> MKIMKEFKEQFGYQLSNFDDMDIKGYANLYQKDIGKDVSMIEQGLKQLSITETEVLLPEQINKKLLGVLNMNEVNQSSNTWVGTLTKQLVSSENNFNIQELPTARKEVFKELLVNRELPQTLRDVITITDDEHVESIPALSYIKDKLATNGIELSLNGSSKYFDRREGHIYTEVADSVVHGSDRTLDDLLKEIFINECVSYETTLLLDKNNASGLIDKDNQDLSLYNQGIKEVSNTSMYDGIKQAMKDIPQTFRRKVSVVMNTEHHDKLIKELAQMGLGTLAGDLTKLFNVSHVVVTDDAQDIFVGDFGHAIYAKYEPIMYNKKKQALKGVYQFALNYVFDIKIVPELLRIVKVK;>MRNFKNDNELLGGNEMPTLYELKQSLGMIGQQLKNKNDELSQKATDPNIDMEDIKQLETEKAGLQQRFNIVERQVQDIEEKEKAKVKDKGEAYQSLSDNEKMVKAKAEFYRHAILPNEFEKPSMEAQRLLHALPTGNDSGGDKLLPKTLSKEIVSEPFAKNQLREKARLTNIKGLEIPRVSYTLDDDDFITDVETAKELKAKGDTVKFTTNKFKVFAAISDTVIHGSDVDLVNWVENALQSGLAAKERKDALAVSPKSGLEHMSFYNGSVKEVEGADMYDAIINALADLHEDYRDNATIYMRYADYVKIISVLSNGTTNFFDTPAEKVF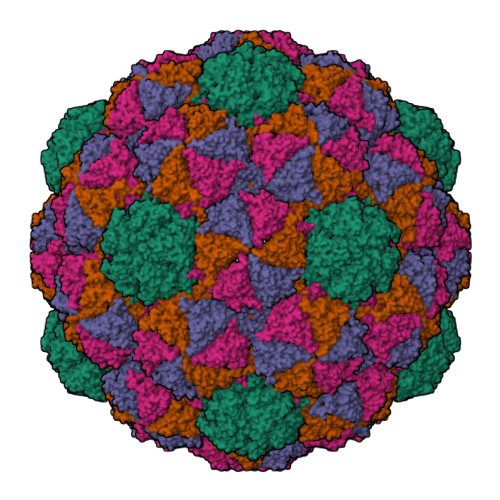GKPVVFTDAAVKPIVGDFNYFGINYDGTTYDTDKDVKKGEYLFVLTAWYDQQRTLDSAFRIAKAKENTGPLPS[3x]> MGSDKIHHHHHHMNNTIPRWRGFNLLEAFSIKSTGNFKEEDFLWMAQWDFNFVRIPMCHLLWSDRGNPFIIREDFFEKIDRVIFWGEKYGIHICISLHRAPGYSVNKEVEEKTNLWKDETAQEAFIHHWSFIARRYKGISSTHLSFNLINEPPFPDPQIMSVEDHNSLIKRTITE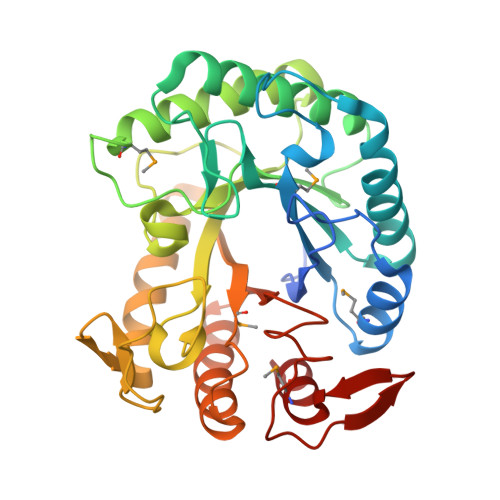IRKIDPERLIIIDGLGYGNIPVDDLTIENTVQSCRGYIPFSVTHYKAEWVDSKDFPVPEWPNGWHFGEYWNREKLLEHYLTWIKLRQKGIEVFCGEMGAYNKTPHDVVLKWLEDLLEIFKTLNIGFALWNFRGPFGILDSERKDVEYEEWYGHKLDRKMLELLRKY>G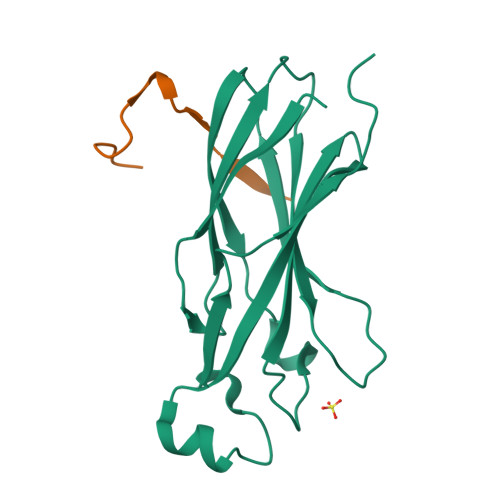AMSIVSLLGIKVLNNPAKFTDPYEFEITFECLESLKHDLEWKLTYVGSSRSLDHDQELDSILVGPVPVGVNKFVFSADPPSAELIPASELVSVTVILLSCSYDGREFVRVGYYVNNEYDEEELRENPPAKVQVDHIVRNILAEKPRVTRFNIVWDNE[4x];>SKKVKRAKLDQTSKGPENLQFS[4x]One element of this ATP requirement is enforced by the nonessential U2 snRNP protein Cus2 (human homolog Tat-SF1), because splicing extracts from Cus2-depleted cells can form pre-spliceosomes in the absence of ATP. Tat-SF1, the human homolog of Cus2, associates with the U2 snRNP and has recently been shown to bind the U2 snRNP protein SF3b1 through a U2AF homology motif (UHM) in Tat-SF1 and a U2AF ligand motif (ULM) in SF3b1. UHMs adopt an RNA recognition motif (RRM)-like fold but have diverged in ways such that they no longer bind RNA, but rather interact with ULMs. Here, we show that Cus2 contains a conserved UHM (U2AF homology motif) that binds Hsh155, the yeast homolog of human SF3b1, through a conserved ULM (U2AF ligand motif).

To view in detail, the interaction between the Hsh155 ULM and one of its binding partner UHMs, we determined a 2.0 Å resolution structure of Tat-SF1 bound to the Hsh155 ULM (residues 98–112). Considering its high binding affinity for the Hsh155 ULM and sequence similarity (55%) to the Cus2 UHM, the Tat-SF1 UHM offers a readily crystallized model system for studying Cus2 UHM-Hsh155 ULM interactions. The Hsh155 ULM is bound to the characteristic α-helical surface of the Tat-SF1 UHM and has well-defined electron density. The positions of the characteristic UHM and ULM residues are conserved. The Hsh155 R100-W101 residues, respectively, interact with Tat-SF1 E286 (Cus2 D204) in the acidic UHM α-helix and F337 (Cus2 F253) of the UHM “RXF” motif, in agreement with the importance of these residues for Cus2–Hsh155 association. In a similar manner as T296-P297 of the SF3b1 ULM4, the C-terminal K104 of the Hsh155 ULM is stacked against the Tat-SF1 W336 side chain. These consistent conformations of the Hsh155 ULM and SF3b1 ULM4 suggest that an extended interface between the C-terminal ULM residues and the “RXF” motif is a shared feature of the Tat-SF1 and Cus2 UHM. A nearby Cus2 aspartate (D201) is likely to account for the additional arginine (R95) at the N-terminus of the Hsh155 ULM, which is disordered in the Tat-SF1-bound structure. The structure of the UHM of Tat-SF1 and the ULM of Hsh155 suggests several features that could explain the higher binding affinity of the Hsh155-Cus2 interaction compared to SF3b1–Tat-SF1 complexes, including (i) an intermolecular Cus2 D254–Hsh155 R100 salt bridge as opposed to the intramolecular SF3b1 interaction (e.g. ULM4 E295–R292), (ii) cation-π stacking and hydrogen bond formation between Hsh155 K104 and Cus2 Y252, and (iii) additional salt bridges between Cus2 D201/D204 and Hsh155 R95. Altogether, we conclude that the ULM of Hsh155 binds to the Tat-SF1 UHM in the characteristic fashion observed for other examples of this protein interaction motif, and the structural similarity between Tat-SF1 and Cus2 provides a detailed model for the molecular basis of Cus2 UHM binding to the ULM of Hsh155.

> MRHERVVIIKNMFHPMDFEDDPLVLNEIREDLRVECSKFGQIRKLLLFDRHPDGVASVSFRDPEEADYCIQTLDGRWFGGRQITAQAWDGTTDY;> SRWDVK>[2x]HMFTG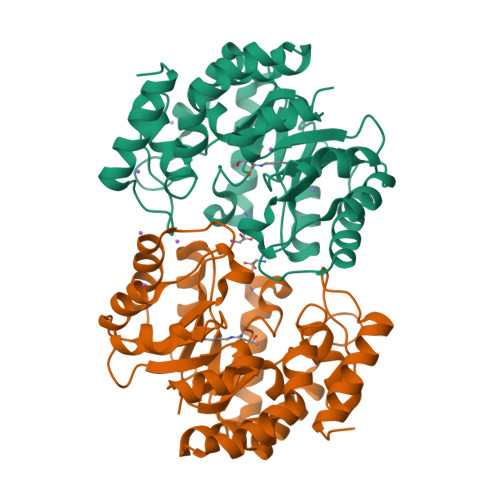SIVAIVTPMDEKGNVCRASLKKLIDYHVASGTSAIVSVGTTGESATLNHDEHADVVMMTLDLADGRIPVIAGTGANATAEAISLTQRFNDSGIVGCLTVTPYYNRPSQEGLYQHFKAIAEHTDLPQILYNVPSRTGCDLLPETVGRLAKVKNIIGIXEATGNLTRVNQIKELVSDDFVLLSGDDASALDFMQLGGHGVISVTANVAARDMAQMCKLAAEGHFAEARVINQRLMPLHNKLFVEPNPIPVKWACKELGLVATDTLRLPMTPITDSGRETVRAALKHAGLL>[2x]MSGAPPPSSGFAPRSYGQQPLSHAPRSSMMSVEYDGIPLPPPSIRSCGSQQYVTSYIPTGAAFPPSSVQDMISSMKSYASATDLVRTYSEIPSVEEALSTLDRAAAALNARRYRDALKLYLEGGYAMANVAERQANPKICNLLTSKGFETLNWCAR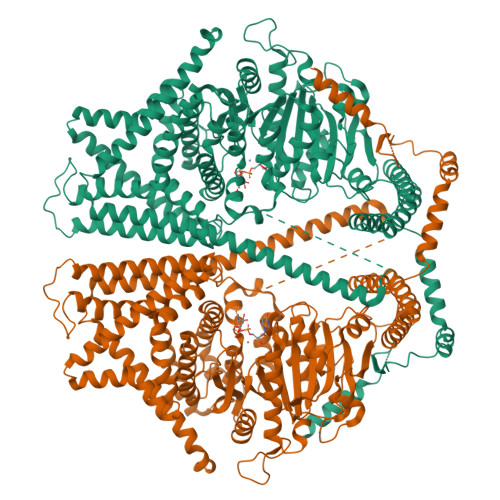LCDWIEGRIKEKHPRPGVHKVGIPVSNWDEDWVGPFMDEEEARRMWYTPVYCPHPIDFSNLGYRLRCVETGRRPRLMICITMYNEGPQQLKATLKKLANNLAYLKEQMPGDEKSLTGAFAGDDVWQNVLVCIVADGREQVHPKTLDYLEAIGLYDEDLLTINSAGIGAQCHLFEHTLQLSVNGKCLLPIQTVFALKENKASKLDSHHWYFNAFAEQIQPEYTAVMDVGTMLTKSALYHLLFAFERNHQIGGACGQLTVDNPFENLSNWVISAQHFEYKISNILDKSLESCFGFISVLPGAFSAYRYEAIRGAPLDAYFQTLNIELDVLGPFIGNMYLAADRILSFEVVARKNCNWTMHYVKDAVARTDVPHDLVGLISQRKRWLNGAFFATLFSIWNWGRIYSESKHTFVRKMAFLVFYVYHLLYTAFGFFLPANLYLALFFIVFQGFQQNRLEFIDTSEYSQTVLDCAVYIYNFSYLFGLLMLIIIGLGNNPKHMKLTYYFVGAVFGLMMMLSSLVGAGIFFSTPATVHSIVVSILTVGVYFIASALHGEVHHIFMTFTHYTALIPSFVNIFTIYSFCNLQDLSWGTKGLHDDPLLAASLDETEKGDFKDVIAKRRALEELRREEKERVENRKKNFEAFRTNVLLTWAFSNLIFALFVVYFASSSTYMPVLYIFVASLNTCRLLGSIGHWVYIHTEGLRGRVIDKSECGNGTGRYPQNSYVQLEEHYAALAEDQRTYASGRTNASVRTVNDVSSAA3-(1H-indazol-4-yl{2-[(1-methyl-1H-indazol-5-yl)amino]pyrimidin-4-yl}amino)propan-1-ol 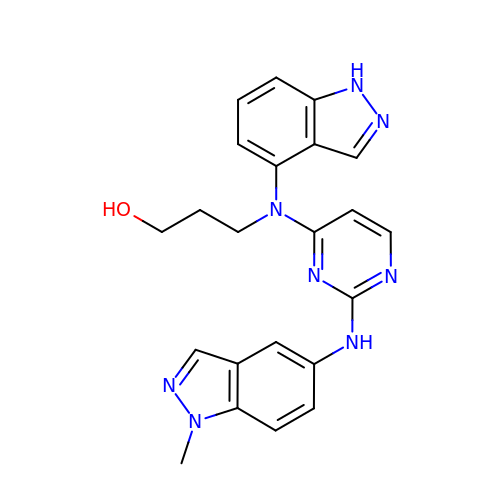| C22 H22 N8 O | VKBDFJNINXDOJC-UHFFFAOYSA-N>[2x]GAMAPATVNVEVLQDKLDHPWALAFLPDNHGMLITLRGGELRHWQAGKGLSAPLSGVPDVWAHGQGGLLDVVLAPDFAQSRRIWLSYSEVGDDGKAGTAVGYGRLSDDLSKVTDFRTVFRQMPKLSTGNHFGGRLVFDGKGYLFIALGENNQRPTAQDLDKLQGKLVRLTDQGEIPDDNPFIKESGVRAEIWSYGIRNPQGMAMNPWSNALW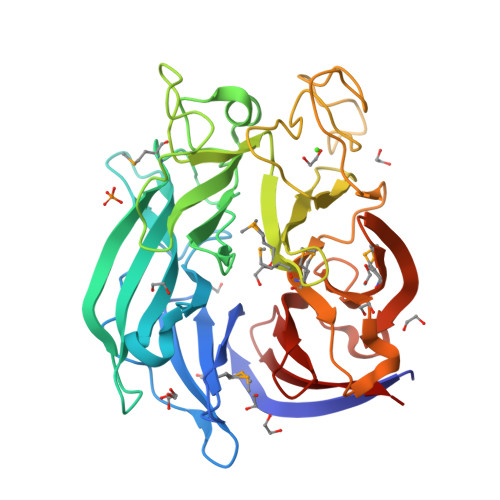LNEHGPRGGDEINIPQKGKNYGWPLATWGINYSGFKIPEAKGEIVAGTEQPVFYWKDSPAVSGMAFYNSDKFPQWQQKLFIGALKDKDVIVMSVNGDKVTEDGRILTDRGQRIRDVRTGPDGYLYVLTDESSGELLKVSPR> TFAYKIDGNEVIFTLWAPYQKSVKLKVLEKGLYEMERDEKGYFTITLNNVKVRDRYKYVLDDASEIPDPASRYQPEGVHGPSQIIQESKEFNNETFLKKEDLIIYEIHVGTFTPEGTFEGVIRKLDYLKDLGITAIEIMPIAQFPGKRDWGYDGVYLYAVQNSYGGPEGFRKLVDEAHKKGLGVILDVVYNHVGPEGNYMVKLGPYFSQKYKTPWGLTFNFDDAESDEVRKFILENVEYWIKEYNVDGFRLDAVHAIIDTSPKHILEEIADVVHKYNRIVIAESDLNDPRVVNPKEKVGYNIDAQWVDDFHHSIHAYLTGERQGYYTDFGNLDDIVKSYKDVFVYDGKYSNFRRKTHGEPVGELDGCNFVVYIQNHDQVGNRGKGERIIKLVDRESYKIAAALYLLSPYIPMIFMGEEYGEENPFY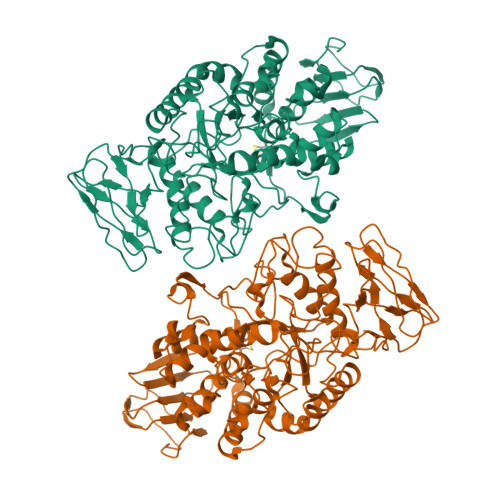FFSDFSDSKLIQGVREGRKKENGQDTDPQDESTFNASKLSWKIDEEIFSFYKILIKMRKELSIACDRRVNVVNGENWLIIKGREYFSLYVFSKSSIEVKYSGTLLLSSNNSFPQHIEEGKYEFDKGFALYKL> MSADHDHDHDHDHDHKPAPMVEEVSDFEILEMAVRELAIEKGLFSAEDHRVWKDYVHTLGPLPAARLVAKAWLDPEYKKLCIEDGVEASKAVGVNWVTSPPTQFGTPSDYCNLRVLADSPTLKHVVVCTLCSCYPRPILGQSPEWYRSPNYRRRLVRWPRQVLAEFGLQLPSEVQIRVADSNQKT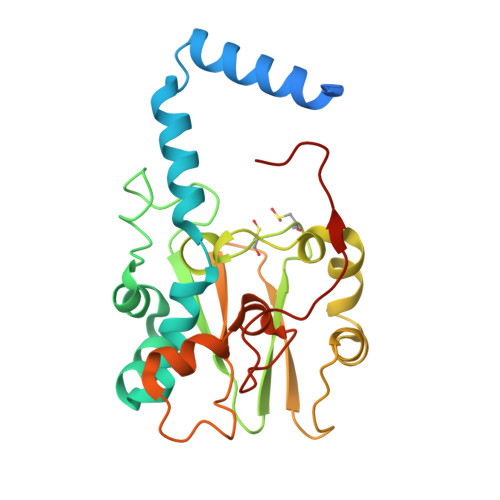RYIVMPVRPEGTDGWTEDQLAEIVTRDCLIGVAVPKPGITVNAKRPVLKANRPVHHDH> RTLDSHASRMTQLK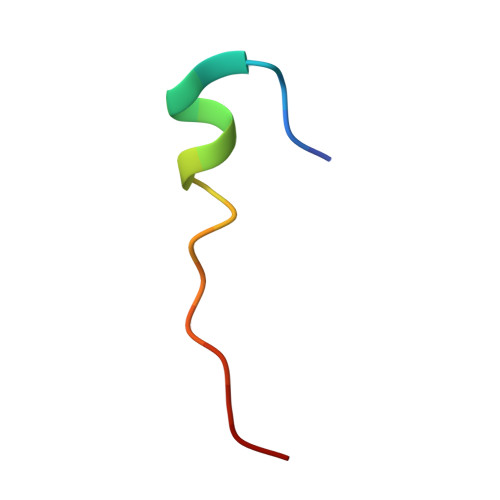KQAAL>MLSLGLEDKVIVVTGGNRGIGAAIVKLLQEMGAKVAFTDLATDGGNTEALGVVANVTDLESMTAAAAEITDKLGPVYGVVANAGITKDNFFPKLTPADWDAVLNVNLKGVAYSIKPFIEGMYERKAGSIVAISSISGERGNVGQTNYSATKAGVIGMMKSLAREGARYGVR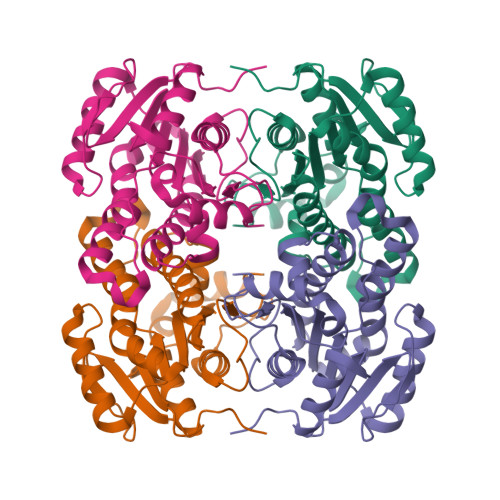ANAVAPGFIDTEMTLAIREDIREKITKEIPFRRFGKPEEIAWAVAFLLSPVASSYVTGEVLRVNGAHHT[3x]>GSQENQMTTQPARIAVTGEGMMTASPDMAILNLSVLRQAKTAREAMTANNEAMTKVLDAMKKAGIEDRDLQTGGIDIQPIYVYPDDKNNLKEPTITGYSVSTSLTVRVRELANVGKILDESVTLGVNQGGDLNLVNDNPSAVIN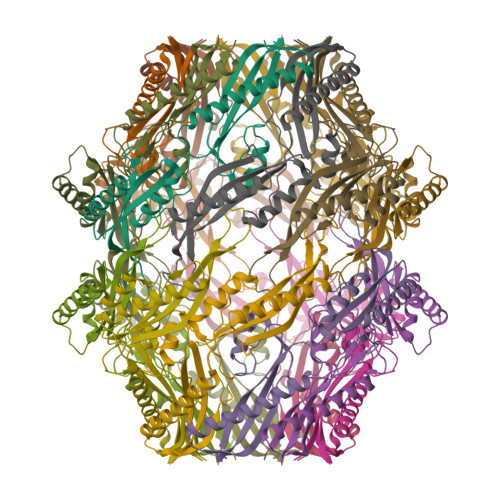EARKRAVANAIAKAKTLADAAGVGLGRVVEISELSRPPMPMPIARGQFRTMLAAAPDNSVPIAAGENSYNVSVNVVFEIK[4x]>MDWSHPQFEKKKKAEWPRKLRSQEWYGGTSRDVIYHRGWLKNQGYPHDLFDGRPVIGILNTWSDMTPCNGHLRELAEKVKAGVWEAGGFPLEVPVFSASENTFRPTAMMYRNLAALAVEEAIRGQPMDGCVLLVGCDKTTPSLLMGAASCDLPSIVVTGGPMLNGYFRGERVGSGTHLWKFSEMVKAGEMTQAEFLEAEASMSRSSGTCNTMGTASTMASMAEALGMALSGNAAIPGVDSRRKVMAQLTGRRIVQMVKDDLKPSEIMTKQAFENAIRTNAAIGGSTNAVIHLLAIAG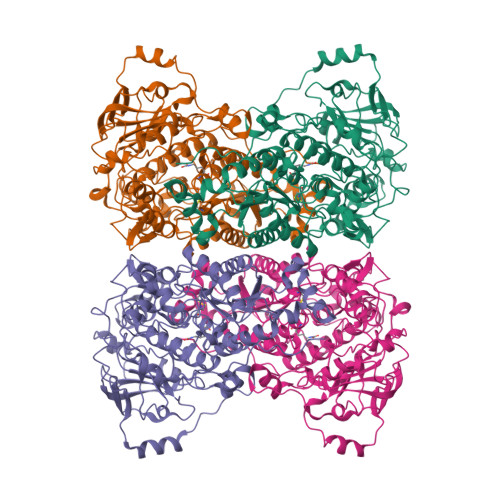RVGIDLSLDDWDRCGRDVPTIVNLMPSGKYLMEEFFYAGGLPVVLKRLGEAGLLHKDALTVSGETVWDEVKDVVNWNEDVILPAEKALTSSGGIVVLRGNLAPKGAVLKPSAASPHLLVHKGRAVVFEDIDDYKAKINDDNLDIDENCIMVMKNCGPKGYPGMAEVGNMGLPPKVLKKGILDMVRISDARMSGTAYGTVVLHTSPEAAVGGPLAVVKNGDMIELDVPNRRLHLDISDEELARRLAEWQPNHDLPTSGYAFLHQQHVEGADTGADLDFLKGCRGNAVGKDSH[2x]> QPIFLNVLEAIEPGVVCAGHDNNQPDSFAALLSSLNELGERQLVHVVKWAKALPGFRNLHVDDQMAVIQYSWMGLMVFAMGWRSFTNVNSAMLYFAPDLVFNEYRMHKSRMYSQCVRMRHLSQEFGWLQITPQEFLCMKALLLFSIIPVDGLKNQKFFDELRMNYIKELDRIIACKRKNP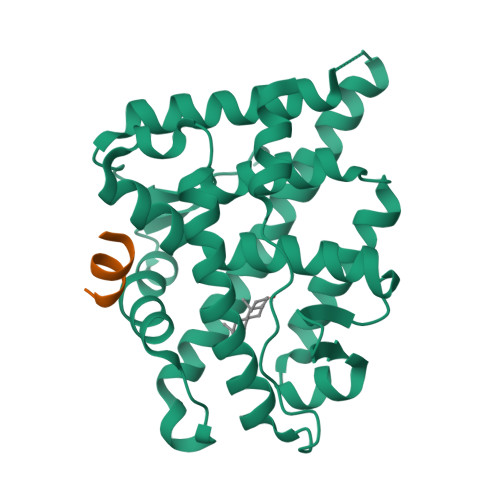TSCSRRFYQLTKLLDSVQPIARELHQFTFDLLIKSHMVSVDFPEMMAEIISVQVPKILSGKVKPIYFHTQ;> ANSSFRDWYTSS> MDLPYYHGCLTKRECEALLLKGGV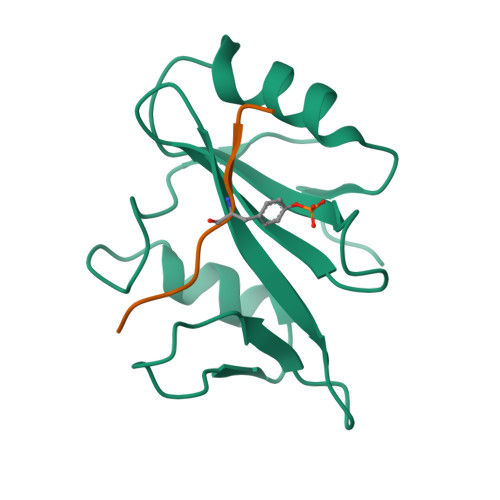DGNFLIRDSESVPGALCLCVSFKKLVYSYRIFREKHGYYRIETDAHTPRTIFPNLQELVSKYGKPGQGLVVHLSNPIMR;> VEKKSLTIYAQVQK Human topoisomerase II beta (TOP2B) modulates DNA topology using energy from ATP hydrolysis. The N-terminal half of the ATPase domain contains the ATP-binding site and is directly involved in clamp closure, undergoing dimerization upon ATP binding. The C-terminal half of the ATPase domain forms the transducer domain, which connects the ATPase domain to the enzyme core (Oestergaard et al., 2004). A heart-shaped dimer is formed with a central cavity that is 31 Å high and 23 Å wide, the dimensions of which cannot easily accommodate a DNA duplex. Each TOP2B ATPase protomer folds into two discrete structural modules: the N-terminal GHKL domain and the C-terminal transducer domain (colored yellow and orange respectively in Figure 2A).

The final TOP2B:AMPPNP model contains residues 46–429 and was refined to a Rwork factor of 19.2% and an Rfree of 23.2%. The adenine ring of AMPPNP is held in place through direct hydrogen bonding with the carbonyl of N136, and stabilization of the ribose sugar is achieved via hydrogen bonding to the hydroxyl group of S165. Hydrogen bonds are made to the α and β phosphate groups of AMPPNP by the side chains of residues N107 and K184, and S164 and N166 respectively. The side chains of Q392 and K394 from the QTK loop of the transducer domain hold the γ phosphate firmly in place, with the switch lysine, K394, forming a salt bridge that is believed to stabilize the transition state of the hydrolysis reaction. The γ phosphate also forms an additional four hydrogen bonds with the main chain of residues R178, N179, Y181, and G182. The catalytic Mg2+ ion is coordinated by a conserved asparagine residue (N107), all three phosphates of AMPPNP, and two water molecules, one of which becomes activated by the catalytic glutamate residue (E103). The key catalytic residue in TOP2B, E103, forms a hydrogen bond to one of the two water molecules coordinated to Mg2+, which activates the water to allow nucleophilic attack on the γ phosphate of ATP. Our data show that the ATPase domain of human TOP2B in complex with AMPPNP is in the restrained conformation with the nucleotide-binding site sequestered from solvent.

> SVERVYQKKTQLEHILLRPDTYIGSVEPLTQFMWVYDEDVGMNCREVTFVPGLYKIFDEILVNAADNKQRDKNMTCIKVSIDPESNIISIWNNGKGIPVVEHKVEKVYVPALIFGQLLTSSNYDDDEKKVTGGRNGYGAKLCNIFSTKFTVETACKEYKHSFKQTWMNNMMKTSEAKIKHFDGEDYTCITFQPDLSKFKMEKLDKDIVALMTRRAYDLAGSCRGVKVMFNGKKLPVNGFRSYVDLYVKDKLDETGVALKVIHELANERWDVCLTLSEKGFQQISFVNSIATTKGGRHVDYVVDQVVGKLIEVVKKKNKAGVSVKPFQVKNHIWVFINCLIENPTFDSQTKENMTLQPKSFGSKCQLSEKFFKAASNCGIVESILNWVKFKAQTQLNKKCS>[2x]MGSSHHHHHHSSGRENLYFQGMATITLERDGLQLVGTREEPFGEIYDMAIIFHGFTANRNTSLLREIANSLRDENIASVRFDFNGHGDSDGKFENMTVLNEIEDANAILNYVKTDPHVRNIYLVGHSQGGVVASMLAGLYPDLIKKVVLLAPAATLKGDALEGNTQGVTYNPDHIPDRLPFKDLTLGGFYLRIAQQLPIYEVSAQFTKPVCLIHGTDDTVVSPNASKKYDQIYQNSTLHLIEGADHCFSDSYQKNAVNLTTDFLQNNNAF

We previously showed that LJ0536, a cinnamoyl esterase purified from L. johnsonii N6.2, is active towards a variety of substrates including short acyl chain aliphatic esters and phenolic esters. The structure showed a canonical α/β fold characteristic of esterases, and the enzyme is dimeric. Two classical serine esterase motifs (GlyXSerXGly) can be recognized from the amino acid sequence, and the structure revealed that the catalytic triad of the enzyme is formed by Ser106, His225, and Asp197, while the other motif is non-functional. The structure revealed a prominent inserted α/β subdomain of 54 amino acids, from which multiple contacts to the aromatic acyl groups of the substrates are made.

The apo-LJ0536 structure was crystallized in the presence of protease, which facilitated successful crystal growth (the mutant Ser106Ala was also crystallized in the presence of protease). The resulting fragment included a loss of four C-terminal residues, such that nearly the entire full-length protein was visible in the electron density map (1–245, plus the five residues from the expression tag). The asymmetric unit of the apo-LJ0536 crystal contained two protein molecules that formed an extensive interface. This interface is formed by α4, α6, and β1. As calculated by the PDBe PISA (Protein Interactions, Surfaces, Assemblies) server, which identifies interfaces between proteins by measuring their buried surface area, the dimer interface comprises 34 and 37 residues of chain A and chain B, respectively, burying a total of 2373 Å2 between the two chains. The interface is primarily hydrophobic (18/37 residues from chain B), although there are six salt-bridges as well. Due to these characteristics, this interface is presumed to be the dimer interface of the protein. The presumed catalytic pocket resembles an open canal-like feature, which has the shape of a boomerang that ends in a hydrophobic pocket buried between the α5 and α6 of the inserted α/β subdomain. Overall, we observed no appreciable differences in the backbone structure between the apo wild-type (WT) enzyme and the Ser106Ala mutant (RMSD of 0.33 Å over all 244 Cα atoms). The inserted α/β subdomain of LJ0536 adopts the same conformation in the apo and ligand-bound structures, suggesting that this is a rigid structure.>[3x]PPGPPGPPGP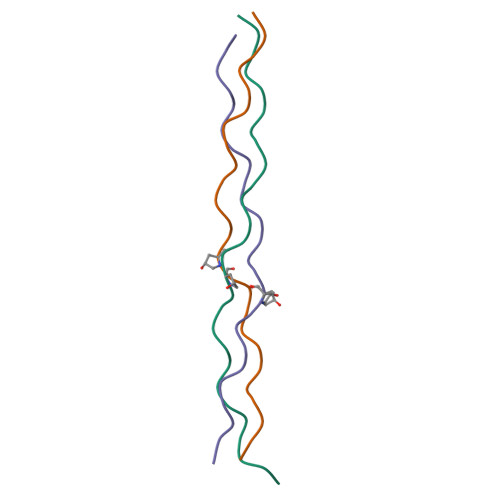PGPDGPPGPPGPPGPPG> PIVNLQAGGRSWKAVESVVFQQLQTVAMQHGLVSEDFERQLAYYATTWTSKDILEVLAMMPGNRAQKELIQGKLNEEAERWVRQNPPGPNVLTVDQIMGVGQTNQQASQANMDQARQICLQWV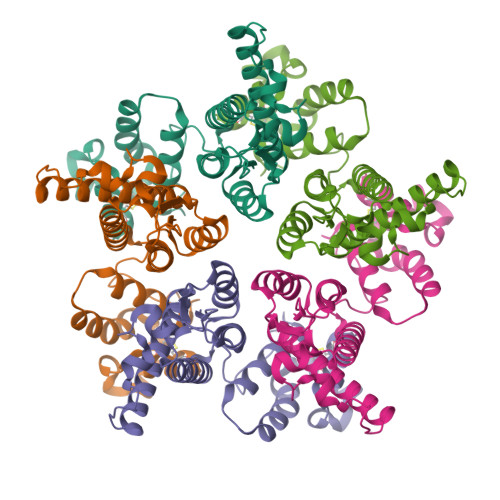ITALRSVRHMSHRPGNPMLVKQKNTESYEDFIARLLEAIDAEPVTDPIKTYLKVTLSYTNASTDCQKQMDRTLGTRVQQATVEEKMQACRDVGSEGFGSSHHHHHH>GMSVPQRPHQFVLTLSCPSAAGQVAAVVGLLDRHRCYVDELTVFDDDLSARFFVRCVFHATDDADALRVDALRREFEPIAERFRMQWAIHDVAA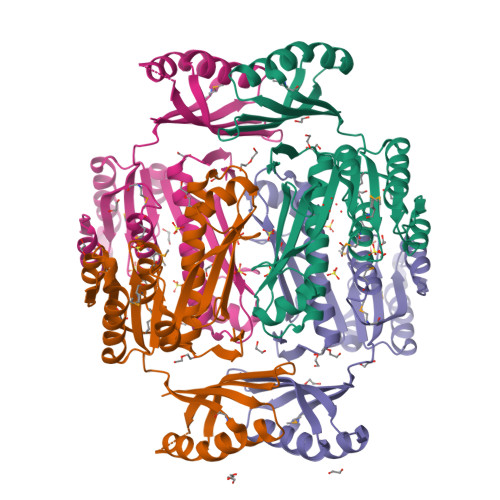RPKVLIMVSKLEHCLADLLFRWKMGELKMDIVGIVSNHPDFAPLAAQHGLPFRHFPITADTKAQQEAQWLDVFETSGAELVILARYMQVLSPEASARLANRAINIHHSFLPGFKGAKPYHQAHARGVKLIGATAHFVTDDLDEGPIIEQVVERVDHSYRPEQLLAVGRDVECITLARAVKAFIERRVFLNGDRTVVFQ[4x]>SMSFPKGFLWGAATASYQIEGAWNEDGKGESIWDRFTHQKGNILYGHNGDIACDHYHRFEEDVLLMKELGLKAYRFSIAWTRIFPDGFGNVNQKGLEFYDRLINKLVENGIEPVITIYHWDLPQKLQDIGGWANSEIVNYYFDYAMLVINRYKDRVKYWITFNEPYCIAFLGHWHGVHAPGIKDFKVAIDVVHNIMLSHFKVVKAVKENNIDVEVGITLNLTPVYLQTERLGYKVSEIEREMVNLSSQLDNELFLDPVLKGNYPQKLFDYLVQKDLLEAQKALSMQQEVKENFIFPDFLGINYYTRAVRLYDENSSWIFPIRWEHPAGEYTEMGWEVFPQGLFDLLMWIKENYPQIPIYITENGAAYNDIVTEDGKVHDSKRIEYLKQHFDQA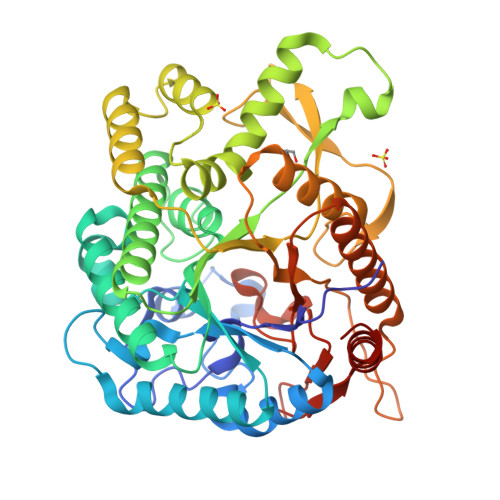RKAIENGVDLRGYFVWSLMDNLEWAMGYTKRFGIIYVDYETQKRIKKDSFYFYQQYIKENS[12x]>[2x]ITLLTLIKTAEHWARQDIRTIEDSKLRALLTLCAVMTRKFSKSQLSLLCETHLRREGLGQDQAEPVLEVYQRLHSDKGGSFEAALWQQWDRQSLIMFITAFLNIALQLPCES;>[2x]TPTVAPPAPVYR

Viral protein 30 (VP30) proteins are present in all filoviruses and perform several important functions, but homologues are lacking in other negative-sense RNA viruses. Additionally, VP30 binds RNA in the presence of zinc and associates with the viral RNA synthesis machinery, which includes nucleoprotein (NP), VP35, and large (L) protein that contains the enzymatic activities. EBOV VP30 (eVP30) is critical for viral transcription (mRNA synthesis), because it is required for initiation at EBOV NP (eNP), the first gene of the seven gene genome. eVP30 has also been implicated in regulation of co-transcriptional editing of viral glycoprotein mRNAs and in modulation of viral transcription reinitiation. We demonstrate that eVP30 binds directly to eNP.

We generated protein crystals for structure determination using the purified eVP30110–272/eNP600–739 complex. Initial low-resolution diffracting crystals were optimized by in situ proteolysis and resulted in several well-diffracting crystals. In contrast to eVP30/eNP contacts, which are largely similar even though the structures belong to different asymmetric units, the ternary configurations of eVP30 suggest that the eVP30/eNP interaction may not impact eVP30–eVP30 interactions. Residues from eNP that span 600–612 are highly conserved not only across all ebolavirus genus members but also marburgvirus as well. Although PPXP motifs typically form a left-handed turn, in the eNP/eVP30 complex structures, the conformation of this motif does not form the expected polyproline type II helix. Instead, these highly conserved eNP residues make extensive contacts with eVP30 residues in an extended conformation. Although the binding pocket is somewhat shallow, the interaction site displays a shape complementarity (Sc) score of 0.6, which is considered significant. Analysis of the interface reveals that there are seven hydrogen bonds between eVP30 and eNP and a number of hydrophobic contacts, which make up much of the observed total of 1,923 Å2 buried surface area. For example, eVP30 Q203A or R213A or Q229A did not result in loss of binding to eNP WT in the FPA, whereas eVP30 E197A and W230A resulted in a near complete loss of binding. However, our data show that the binding site identified in our structure, which includes residues such as W230, results in complete loss of binding and corresponding loss of activity in viral RNA synthesis.>METLTVHAPSPSTNLPSYGNGAFSLSAPHVPGAGPLLVQVVYSFFQSPNMCLQALTQLEDYIKKHGASNPLTLQIISTNIGYFCNADRNLVLHPGISVYDA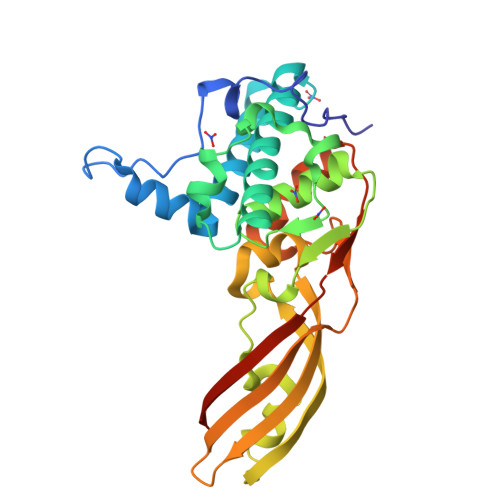YHFAKPAPSQYDYRSMNMKQMSGNVTTPIVALAHYLWGNGAERSVNIANIGLKISPMKINQIKDIIKSGVVGTFPVSTKFTHATGDYNVITGAYLGNITLKTEGTLTISANGSWTYNGVVRSYDDKYDFNASTHRGIIGESLTRLGAMFSGKEYQILLPGEIHIKESGKRAAHHHHHH[2x]> YEASILTHDSSIRYLQEIYNSNNQKIVNLKEKVAQLEAQCQEPCKDTVQIHDITGKDCQDIANKGAKQSGLYFIKPLKANQQFLVYCEIDGSGNGWTVFQKRLDGSVDFKKNWIQYKEGFGHLSPTGTTEFWLGNEKIHLISTQSAIPYALRVELEDWNGRTSTADYAMFKVGPEADKYRLTYAYFAGGDAGDAFDGFDFGDDPSDKFFTSHNGMQFSTWDNDNDK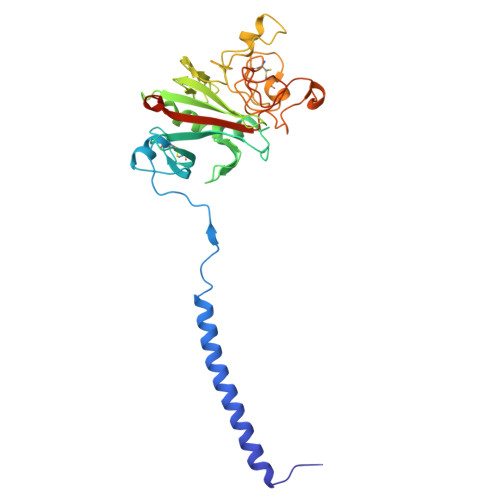FEGNCAEQDGSGWWMNKCHAGHLNGVYYQGGTYSKASTPNGYDNGIIWATWKTRWYSMKKTTMKIIPFNRLTIGEGQQHHLGGAK>SLMADEIAKAQVARPGGDTIFGKIIRKEIPAKIIFEDDRCLAFHDISPQAPTHFLVIPKKHI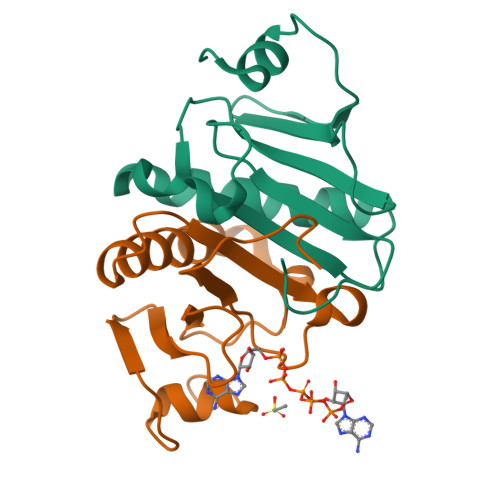SQISVAEDDDESLLGHLMIVGKKCAADLGLNKGYRMVVNEGSDGGQSVYHVHLAVLGGRQMHWPPG[2x]>[4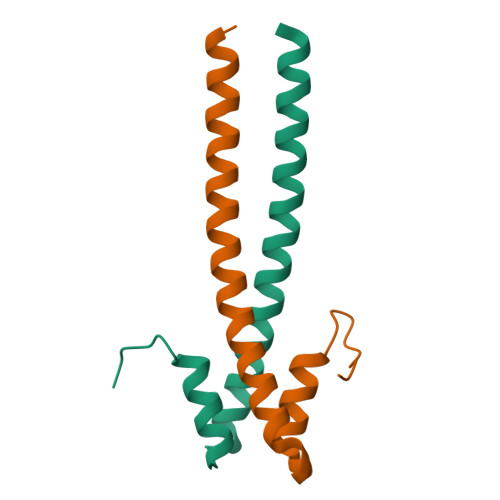x]LSNQKLTKKALIKEYTEEIERLKRDLAALEKERDFYFGKLRNIELICQENEGENDPVLQRIVDILYATDEGFVIPD> GP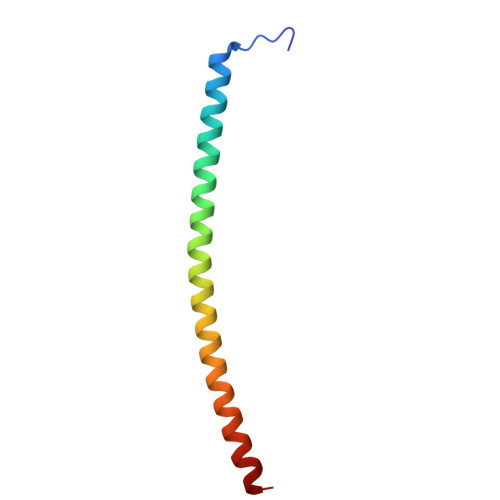GSMQMNEAKIAECLQTISDLETECLDLRTKLCDLERANQTLKDEYDALQITFTALEGKLRKTTEENQ>[4x]GTSRHVFIRTELSFIKNNVPCIRDMFF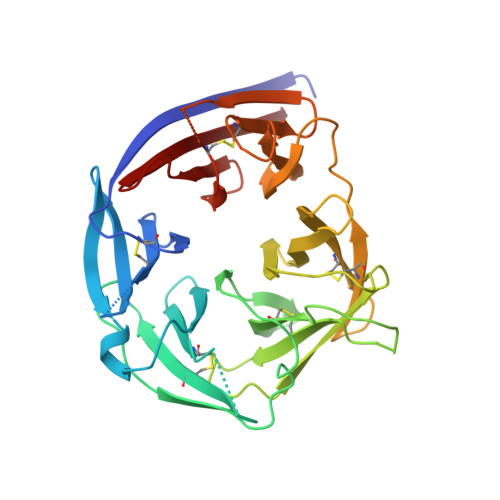IYKRELYNICLDDLKGEEDETHIYVQKKVKDSWITLNDLFKETDLTGRPHIFAYVDVEEIIILLCEDEEFSNRKKDMTCHRFYSNDGKEYNNAEITISDYILKDKLLSSYVSLPLKIENREYFLICGVSPYKFKDDNKKDDILCMASHDKGETWGTKIVIKYDNYKLGVQYFFLRPYISKNDLSFHFYVGDNINNVKNVNFIECTHEKDLEFVCSNRDFLKDNKVLQDVSTLNDEYIVSYGNDNNFAECYIFFNNENSILIKPEKYGNTAAGCYGGTFVKIDENRALFIYSSSQGIYNIHTIYYANYE> SENPFIAHELKQTSVNEITAHVINEPASLKLTTISTILHAPLQNL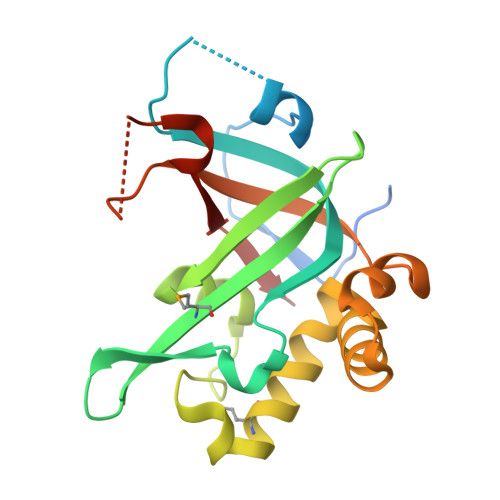LKPRKHRLRVQVVDFWPKSLTQFAVLSQPPSSYVWMFALLVRDVSNVTLPVIFFDSDAAELINSSKIQPCNLADHPQMTLQLKERLFLIWGNLEERIQHHISKGESPTLAAEDVETPWFDIYVKEYIPVIGNTKDHQSLTFLQKRWRGFGTKIV> MIVKHLEEIVDTKDDIDTTTWNSRRLLLTKDGMGFSLNDTLIKAGTETLIWYKNHVEAVYCIEGEGEIEVVGGETYPITPGMMYALDGHEKHYLRARSQMRMVCVFNPPLTGAEVHDEEGTYPLLAPITDNWSHPQFE

While the EctA and EctB enzymes have amino acid sequence-related counterparts in various biochemical pathways in microorganisms, the ectoine synthase (EctC) is considered the diagnostic enzyme for ectoine production. Crystallographic analysis of the psychrophilic S. alaskensis EctC protein [(Sa)EctC] showed that ectoine synthase is a member of the cupin superfamily. By using an ectoine synthase from the thermo-tolerant bacterium P. lautus, we were able to obtain high-resolution crystal structures of the full-length EctC enzyme in complex with its iron-cofactor, its substrate, and its product. The (Pl)EctC protein is a head-to-tail dimer where backbone interactions between two ß-sheets mediate the contacts between the monomers in the dimer assembly.

We were able to obtain a (Pl)EctC crystal structure that contained both the iron ion and an ectoine molecule. After manual rebuilding and several cycles of refinement, the structure of the (Pl)EctC::Fe/ectoine complex was finalized with an R-factor of 18.2%, an Rfree of 24%, and a resolution of 2.5 Å. The ectoine molecule is coordinated within the active site of the (Pl)EctC enzyme through five direct interactions with the following residues: Ser-23, Asn-38, Tyr-52, Glu-57, and Phe-106. Ectoine exhibits a significantly different conformation to that of the bound N-γ-ADABA molecule. In particular, Tyr-52 and Glu-57 are no longer involved in any H-bonding interactions with N1 of ectoine (derived from the amidic N5 of N-γ-ADABA), but now both residues form H-bonds to N3 of ectoine, which is derived from the α-amino group of N-γ-ADABA. These new H-bonds towards N3 of ectoine also appear to be stronger than those formed originally with N-γ-ADABA, as suggested from their shorter distances (3.2 Å to Tyr-52, and 3.7 Å to Glu-57), and are further stabilized by an interaction with Phe-106. In addition, the side-chain of Asn-38 makes a direct contact to the carboxylate of ectoine, and this side chain is in turn held in place through stabilizing interactions with the side-chain of Ser-23. There may also be a direct interaction between the iron and the methyl group of the ectoine molecule. The side chain of Trp-21 adopts a single conformation in the (Pl)EctC::Fe-ectoine structure and thereby provides additional stabilizing contacts to the ectoine ligand (compare Fig. 6a,b). When the crystal structures of the (Pl)EctC::Fe/N-γ-ADABA and the (Pl)EctC::Fe/ectoine complexes are overlaid, it becomes apparent that the substrate (N-γ-ADABA) and the reaction product (ectoine) occupy almost the same position within the (Pl)EctC active site. Hence, the observed mode of ectoine binding indicates the requirement of an extensive conformational change of the linear N-γ-ADABA molecule during enzyme catalysis to yield the spatial position of the cyclic ectoine molecule.>HHHHHHFNLPPGNYKKPKLLYCSNGGHFLRIDPDGTVDGTRDRSDQHIQLQLSAESVGEVYIK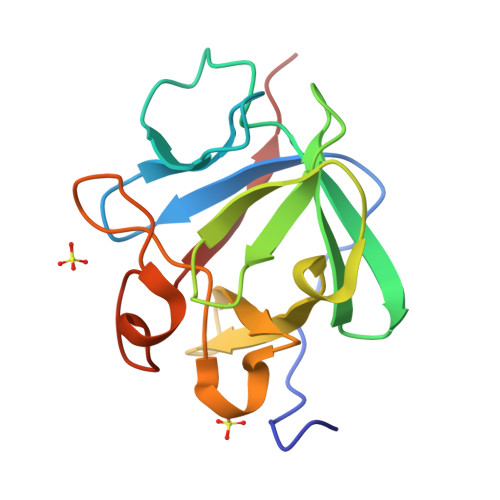STETGQYLAMDTDGLLYGSQTPNEECLFLERLEENHYNTYISKKHAEKNWFVGLKKNGSCKRGPRTHYGQKAILFLPLPVSSD[2x]> MGSSHHHHH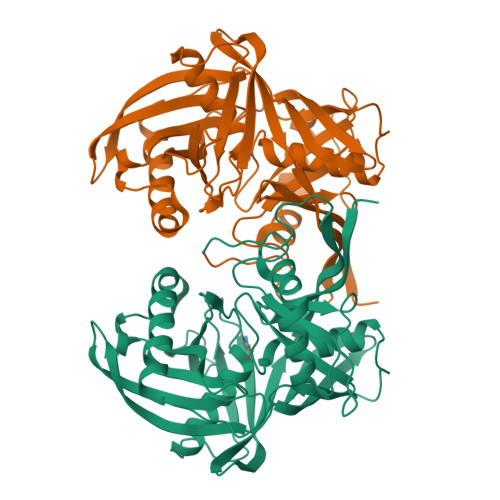HSQDLFADHVFHVVDTHTEGEPTRIVLSGVNVKGEDIIEKREYFKEHYDWIRTALLHEPRGHSDQFGAVLVPSDIADFGVIYMDTSGYLDMCGHATMGVATVLVELGIIEKKEPYTTVKLETPAGLVEAKAKVKGGVVKEVTVVDVPSFYVGEFVIEYPGRGKIKVDVAFGGNFYVIADARDLGLRVRREYIKELIPTALKLIKVANEQIKVQHPRKGVQNRINLAMLTDEPEREDSDGKNVVIWGEGSVDRSPCGTGSASRVATLYSKGILKEGDIFVHESILGTQFRIKIVGTTKIGEYTAIIPEITGSAYITKISQDIISKNDPLWKGFLLR> MVYTNWQSSYTRLFVSKPWMWHPLAWMTLSVGIWWKFGKESLCNERSFYIHTHP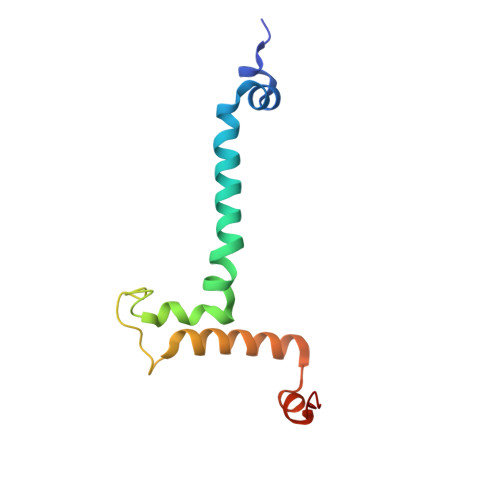KWAPHKFHTVYNWSRDPIKWTLAEQYASIIRNTNTDIEAVLKIKLPANAN> MKHHHHHHPMGLEVLFQGPPRDIALGSSVVSIKNQALGGSLLHSHIQTYPDGSNQQQVTCYGYKDANNEWFFNRERGLPSWSENETDIEYLKPGTSYRLVHKSTGRNLHTHPVA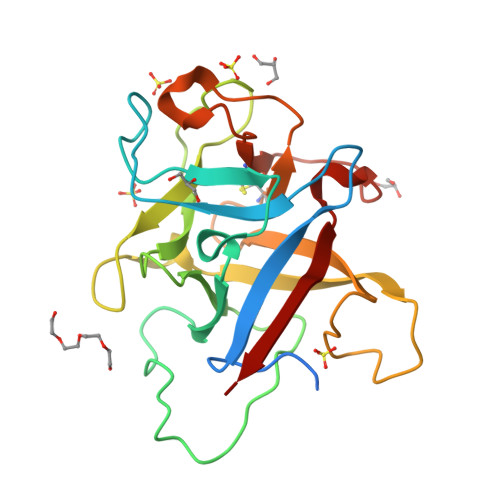APVSKTQWEVSGYGDNVVGDNKDNWVIEIMDQRGDEDPEKLHTLTTSFRIKNLEMGCYLAQTGNSLPEWGFRQQEVVCMKNPFKRDKRTWWNIETHENER>[5x]GGVEVLEVKTGVDAITEVECFLNPEMGDPDENLRGFSLKLSAENDFSSDSPERKMLPCYSTARIPLPNLNEDLTCGNLLMWEAVTVQTEVIGITSMLNLHAGSQKVHE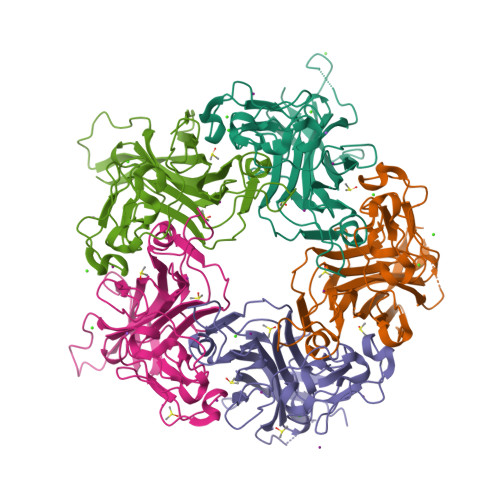HGGGKPIQGSNFHFFAVGGEPLEMQGVLMNYRSKYPDGTITPKNPTAQSQVMNTDHKAYLDKNNAYPVECWVPDPSRNENARYFGTFTGGENVPPVLHVTNTATTVLLDEQGVGPLCKADSLYVSAADICGLFTNSSGTQQWRGLARYFKIRLRKRSVKNPY>[4x]PMSEKQLAEVVERTVTPLMKAQ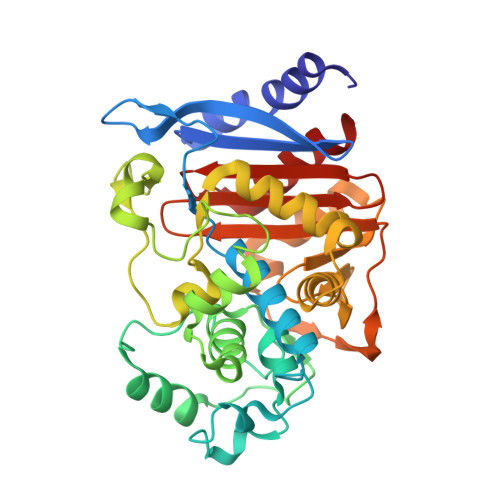AIPGMAVAVIYEGQPHYFTFGKADVAANKPVTPQTLFELGSISKTFTGVLGGDAIARGEISLGDPVTKYWPELTGKQWQGIRMLDLATYTAGGLPLQVPDEVKDNASLLRFYQNWQPQWKPGTTRLYANASIGLFGALAVKPSGMSYEQAITTRVFKPLKLDHTWINVPKAEEAHYAWGYRDGKAVHVSPGMLDAEAYGVKTNVQDMASWVMVNMKPDSLQDNSLRKGLTLAQSRYWRVGAMYQGLGWEMLNWPVDAKTVVEGSDNKVALAPLPAREVNPPAPPVNASWVHKTGSTGGFGSYVAFIPEKQLGIVMLANKSYPNPARVEAAYRILSAL> MVTSEQLLFLEAWRAVDRAYVDKSFNGQSWFKLRETYLKKEPMDRRAQTYDAIRKLLAVLDDPFTRFLEPSRLAALRRGTAGSVTGVGLEITYDGGSGKDVV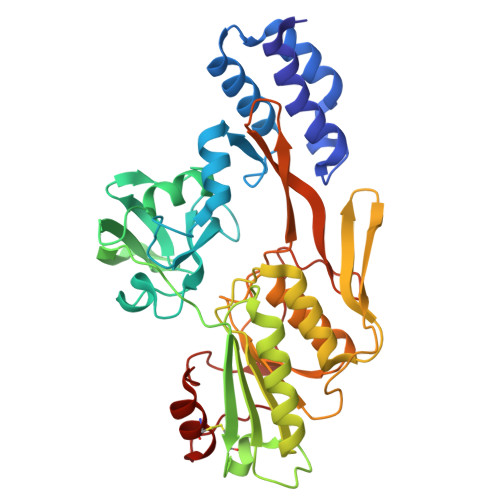VLTPAPGGPAEKAGARAGDVIVTVDGTAVKGLSLYDVSDLLQGEADSQVEVVLHAPGAPSNTRTLQLTRQKVTINPVTFTTCSNVAAAALPPGAAKQQLGYVRLATFNSNTTAAAQQAFTELSKQGVAGLVLDIRNNGGGLFPAGVNVARMLVDRGDLVLIADSQGIRDIYSADGNSIDSATPLVVLVNRGTASASEVLAGALKDSKRGLIAGERTFGKGLIQTVVDLSDGSGVAVTVARYQTPAGVDINKIGVSPDVQLDPEVLPTDLEGVCRVLGSDAAPRLFG> SMKRTYPEPTPIYHITHIDNLKGILRMGKLLAHNQSPPKQRSIAYAHIQERRNRAKVPQPPGGVLHDYVPFYFCPRSPMLYAI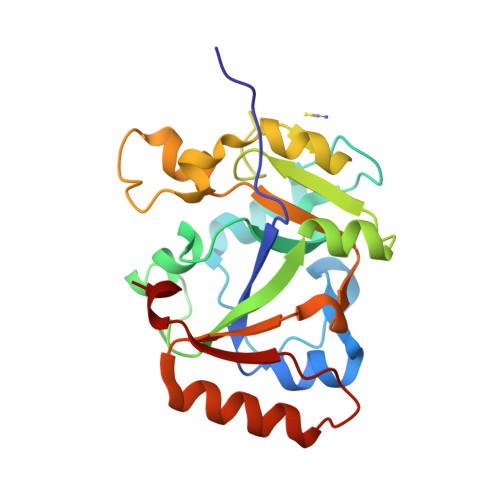YSGATEYQGGQEPILHLVSSAQAVHKAGLPFVFTDRHGVLSHARFFRQLEELAQLDWEAIQASYWADPPELREKKQAAFLVYKAFPWALIEEIAVYSQRVGEEVLKILKQFPEARRPRVCIRKDWYY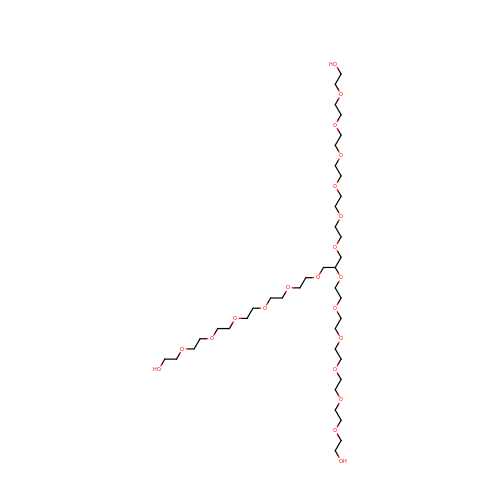Glycerol ethoxylate | C39 H80 O21 | PVDRPYVNUSQYRG-UHFFFAOYSA-N(2S)-propane-1,2-diyl 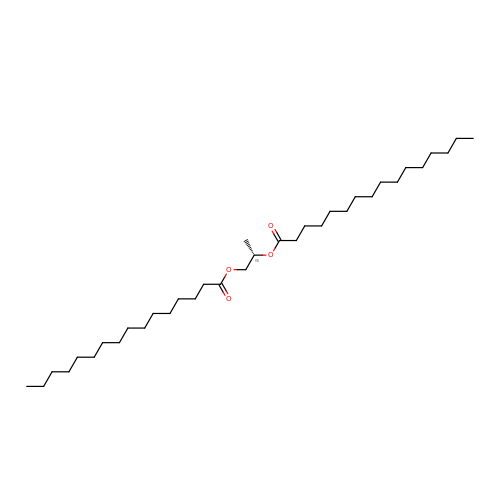dihexadecanoate | C35 H68 O4 | UWTZRBLIYNMYTC-XIFFEERXSA-N>[4x]MHHHHHHSSGLVPRGSLRVGNRYRLGRKIGSGSFGDIYLGTDIAAGEEVAIKLECVKTKHPQLHIESKIYKMMQGGVGIPTIRWCGAEGDYNVMVMELLGPSLEDLFNFCSRKFSLKTVLLLADQMISRIEYIHSKNFIHRDVKPDNFLMGLGKKGNLVYIIDFGLAKKYRDARTHQH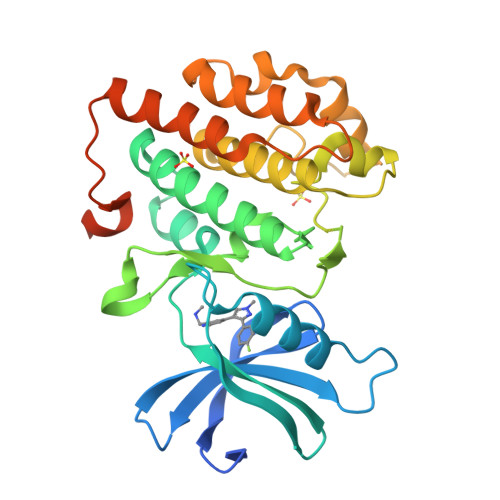IPYRENKNLTGTARYASINTHLGIEQSRRDDLESLGYVLMYFNLGSLPWQGLKAATKRQKYERISEKKMSTPIEVLCKGYPSEFATYLNFCRSLRFDDKPDYSYLRQLFRNLFHRQGFSYDYVFDWNMLKFGASRAADDAERERRDREERLRH>GAHMAGRSMQAARCPTDELSLSNCAVVSEKDYQSGQHVIVRTSPNHKYIFTLRTHPSVVPGSVAFSLPQRKWAGLSIGQEIEVALYSFDKAKQCIGTMTIEIDFLQKKNIDSNPYDTDKMAAEFIQQFNNQAFSVGQQLVFSFNDKLFGLLVKDIEAMDPSILKGEPASGKRQKIEVGLVVGNSQVAFEKAENSSLNLIGKAKTKENRQSIINPDWNFEKMGIGGLDKEFSDIFRRAFASRVFPPEIVEQMGCKHVKGILLYGPPGCGKTLLARQIGKMLNAREPKVVNGPEILNKYVGESEANIRKLFADAEEEQRRLGANSGLHIIIFDEIDAICKQRGSMAGSTGVHDTVVNQLLSKIDGVEQLNNILVIGMTNRPDLIDEALLRPGRLEVKMEIGLPDEKGRLQILHIHTARMRGHQLLSADVDIKELAVETKNFSGAELEGLVRAAQSTAMNRHIKASTKVEVDMEKAESLQVTRGDFLASLENDIKPAFGTNQEDYASYIMNGIIKWGDPVTRVLDDGELLVQQTKNSDRTPLVSVLLEGPPHSGKTALAAKIAEESNFPFIKICSPDKMIGFSETAKCQAMKKIFDDAYKSQLSCVVVDDIERLLDYVPIGPRFSNLVLQALLVLLKKAPPQGRKLLIIGTTSRKDVLQEMEMLNAFSTTIHVPNIATGEQLLEALELLGNFKDKERTTIAQQVKGKKVWIGIKKLLMLIEMSLQMDPEYRVRKFLALLREEGASPLDFD[6x];> SMAEDADMRNELEEMQRRADQLADESLESTRRMLQLVEESKDAGIRTLVMLDEQGEQLERIEEGMDQINKDMKEAEKNLTDLGK

The membrane-anchored SNARE (soluble N-ethylmaleimide-sensitive factor acceptor protein receptor) proteins provide the energy to drive membrane fusion in various cellular contexts, such as intracellular trafficking and exocytosis. Supercomplexes of NSF, α-SNAP, and either a syntaxin tetramer or one of two binary complexes of syntaxin—SNAP-25 reveal atomic details of SNARE processing and show how sequential ATP hydrolysis drives disassembly. NSF comprises three structured domains connected by flexible linkers—the adapter N-domain followed by the D1 and D2 AAA+ domains. Six NSF protomers come together to form the active form of the enzyme, a homo-hexamer.

To gain insight into the structural nature of binary complex formation and disassembly by NSF, we prepared a complex of NSF, ɑ-SNAP, and the binary t-SNARE complex (21bin20S) composed of full-length soluble SNAP-25 and soluble syntaxin-1a (1–267) in the absence of divalent cation (i.e., non-hydrolyzing conditions) and performed single-particle cryo-EM. First, models of the NSF D1 and D2 domains with substrate bound in the D1 pore were built into two high-resolution (2.88 Å, 2.92 Å) classes from a single dataset, differing only in the state of F protomer engagement with substrate. For datasets with particles collected under non-hydrolyzing conditions, NSF is found in two general conformations, primarily differentiated by their F protomer state (left column). Two high-resolution 21bin20S classes from the 2:1 binary SNARE complex dataset reveal large-scale conformational displacement connected to the D1 F protomer nucleotide state and SNARE substrate engagement. The first class is ATP-bound and fully SNARE substrate-engaged, while the second has a nucleotide-free and SNARE substrate-disengaged F protomer. The engagement of F at the top of the ring accompanies a relaxation of A into the split. Otherwise, the classes are nearly identical; protomers B–E D1 domains also bind ATP, while protomer A, at the bottom of the D1 split, is ADP-bound in both cases. Comparison of the two classes reveals limited differences outside of the protomers A and F positions, as the change in protomer F position allows additional relaxation of protomer A into the split. Two states dominate in the absence of Mg2+ (left); the top class (#4) has SNARE substrate disengaged, nucleotide-free protomer F, while the bottom class (#3) has SNARE substrate-engaged, ATP-bound F. With the addition of Mg2+ (middle), E is Mg2+-bound.> MGSSHHHHHHSQDPNSHMKETPLSNCERRFLLRAIEEKKRLDGRQTYDYRNIRISFGTDYGCCIVELGKTRVLGQVSCELVSPKLNRATEGILFFNLELSQMAAPAFEPGRQSDLLVKLNRLMERCLRNSKCIDTESLCVVAGEKVWQIRVDLHLLNHDGNIIDAASIAAIVALCHFRRPDVSVQGDEVTLYTPEERDPVPLSIHHMPICVSFAFFQQGTYLLVDPNEREERVMDGLLVIAMNKHREICTIQSSGGIMLLKDQVLRCSKIAGVKVAEITELILKALENDQKVRKEGGKFGFAESIANQRITAFKMEKAPXXXXXXXXXXXXXXXXXXXXXXXXXXXXXXXXXXXXXXX;> MADPMAGLELLSDQGYRVDGRRAGELRKIQARMGVFAQADGSAYIEQGNTKALAVVYGPHEIRGSRARALPDRALVNCQYSSATFSTGERKRRPHGDRKSCEMGLQLRQTFEAAILTQLHPRSQIDIYVQVLQADGGTYAACVNAATLAVLDAGIPMRDFVCACSAGFVDGTALADLSHVEEAAGGPQLALALLPASGQIALLEMDARLHEDHLERVLEAAAQAARDVHTLLDRVVRQHVREASILLGD;> DPMAAGFKTVEPLEYYRRFLKENCRPDGRELGEFRTTTVNIGSISTADGSALVKLGNTTVICGVKAEFAAPSTDAPDKGYVVPNVDLPPLCSSRFRSGPPGEEAQVASQFIADVIENSQIIQKEDLCISPGKLVWVLYCDLICLDYDGNILDACTFALLAALKNVQLPEVTINEETALAEVNLKKKSYLNIRTHPVATSFAVFDDTLLIVDPTGEEEHLATGTLTIVMDEEGKLCCLHKPGGSGLTGAKLQDCMSRAVTRHKEVKKLMDEVIKSMKPK;> SLMEEETHTDAKIRAENGTGSSPRGPGCSLRHFACEQNLLSRPDGSASFLQGDTSVLAGVYGPAEVKVSKEIFNKATLEVILRPKIGLPGVAEKSRERLIRNTCEAVVLGTLHPRTSITVVLQVVSDAGSLLACCLNAACMALVDAGVPMRALFCGVACALDSDGTLVLDPTSKQEKEARAVLTFALDSVERKLLMSSTKGLYSDTELQQCLAAAQAASQHVFRFYRESLQRRYSKS;> MGSSHHHHHHSQDPMASVTLSEAEKVYIVHGVQEDLRVDGRGCEDYRCVEVETDVVSNTSGSARVKLGHTDILVGVKAEMGTPKLEKPNEGYLEFFVDCSASATPEFEGRGGDDLGTEIANTLYRIFNNKSSVDLKTLCISPREHCWVLYVDVLLLECGGNLFDAISIAVKAALFNTRIPRVRVLEDEEGSKDIELSDDPYDCIRLSVENVPCIVTLCKIGYRHVVDATLQEEACSLASLLVSVTSKGVVTCMRKVGKGSLDPESIFEMMETGKRVGKVLHASLQSVVHKEESLGPKRQKVGFLG;> MPGDHRRIRGPEESQPPQLYAADEEEAPGTRDPTRLRPVYARAGLLSQAKGSAYLEAGGTKVLCAVSGPRQAEGGERGGGPAGAGGEAPAALRGRLLCDFRRAPFAGRRRRAPPGGCEERELALALQEALEPAVRLGRYPRAQLEVSALLLEDGGSALAAALTAAALA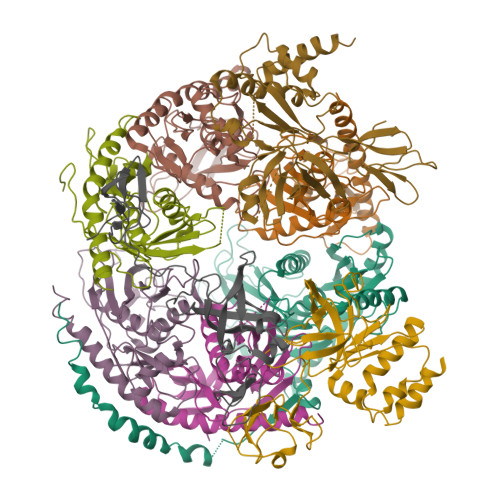LADAGVEMYDLVVGCGLSLAPGPAPTWLLDPTRLEEERAAAGLTVALMPVLNQVAGLLGSGEGGLTESWAEAVRLGLEGCQRLYPVLQQSLVRAARRRGAAAQP;> MGSSHHHHHHSQDPMAEPASVAAESLAGSRARAARTVLGQVVLPGEELLLPEQEDAEGPGGAVERPLSLNARACSRVRVVCGPGLRRCGDRLLVTKCGRLRHKEPGSGSGGGVYWVDSQQKRYVPVKGDHVIGIVTAKSGDIFKVDVGGSEPASLSYLSFEGATKRNRPNVQVGDLIYGQFVVANKDMEPEMVCIDSCGRANGMGVIGQDGLLFKVTLGLIRKLLAPDCEIIQEVGKLYPLEIVFGMNGRIWVKAKTIQQTLILANILEACEHMTSDQRKQIFSRLAES;> MGSSHHHHHHSQDPHMAMEMRLPVARKPLSERLGRDTKKHLVVPGDTITTDTGFMRGHGTYMGEEKLIASVAGSVERVNKLICVKALKTRYIGEVGDIVVGRITEVQQKRWKVETNSRLDSVLLLSSMNLPGGELRRRSAEDELAMRGFLQEGDLISAEVQAVFSDGAVSLHTRSLKYGKLGQGVLVQVSPSLVKRQKTHFHDLPCGASVILGNNGFIWIYPTPEHKEEEAGGFIANLEPVSLADREVISRLRNCIISLVTQRMMLYDTSILYCYEASLPHQIKDILKPEIMEEIVMETRQRLLEQEG;> MGSSHHHHHHSQDPMAPPVRYCIPGERLCNLEEGSPGSGTYTRHGYIFSSLAGCLMKSSENGALPVVSVVRETESQLLPDVGAIVTCKVSSINSRFAKVHILYVGSMPLKNSFRGTIRKEDVRATEKDKVEIYKSFRPGDIVLAKVISLGDAQSNYLLTTAENELGVVVAHSESGIQMVPISWCEMQCPKTHTKEFRKVARVQPEFLQT> MNSEYDYLFKLLLIGNSGVGKSCLLLRFSDDTYTNDYISTIGVDFKIKTVELDGKTVKLQIWDTAGQERFRTITSSYYRGSHGIIIVYDVTDQESFNGVKMWLQEIDRYATSTVLKLLVGNKCDLKDKRVVEYDVAKEFADANKMPFLETSALDSTNVEDAFLTMARQIKESMSQQNLN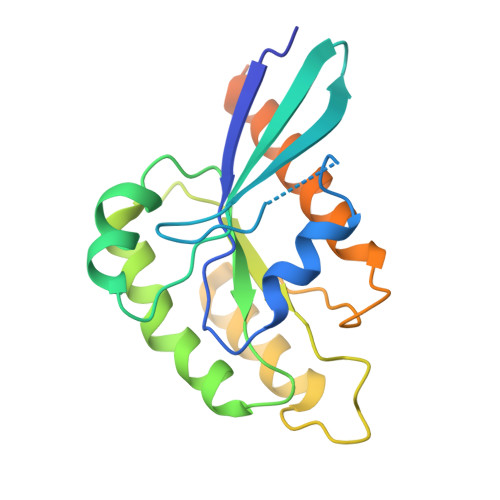ETTQKKEDKGNVNLKGQSLTNTGGGCC>[3x]MSVCHKHSVIGVLDSGVGGLTVASEIIRQLPKESICYIGDNERCPYGPRSVEEVQSFVFEMVEFLKQFPLKALVVACNTAAAATLAALQEALSIPVIGVIHPGARAAIKVT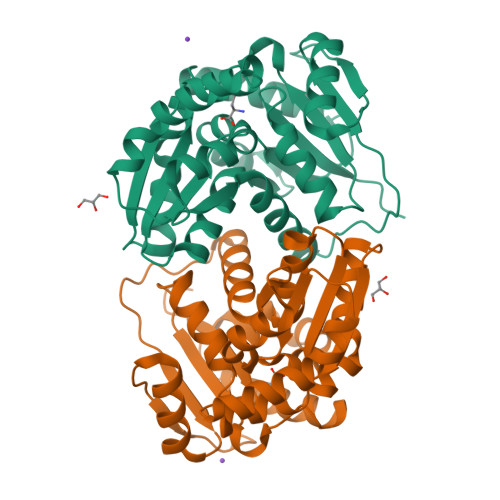KKGKIGVIGTVGTIQSNMYEKALHELDTYLKVHSHACPTLATVVENRLEDTAYVTQQVKQALLPLTKEDIDTLILGCTHYPLLESYIKKELGEDVTIISSAEETAIELSTILQHKGILADNLNPKHRFFTTGSVSSFEHIAERWLGYQISVDCVDLPVKNARICN>MGHHHHHHAENLYFQGHMLRLSAPGQLDDDLCLLGDVQVPVFLLRLGEASWALVEGGISRDAELVWADLCRWVADPSQVHYWLITHKHYDHCGLLPYLCPRLPNVQVLASERTCQAWKSESAVRVVERLNRQLLRAEQRLPEACAWDALPVRAVADGEWLELGPRHRLQVIEAHGHSDDHVVFYDVRRRRLFCGDALGEFDEAEGVWRPLVFDDMEAYLESLERLQRLPTLLQLIPGHGGLLRGRLAADGAESAYTECLRLCRRLLWRQSMGESLDELSEELHRAWGGQSVDFLPGELHLGSMRRMLEILSRQALPLD[2x];>[2x]MRNDGGFLLWWDGLRSEMQPIHDSQGVFAVLEKEVRRLGFDYYAYGVRHTIPFTRPKTEVHGTYPKAWLERYQMQNYGAVDPAILNGLRSSEMVVWSDSLFDQSRMLWNEARDWGLCVGATLPIRAPNNLLSVLSVARDQQNISSFEREEIRLRLRCMIEL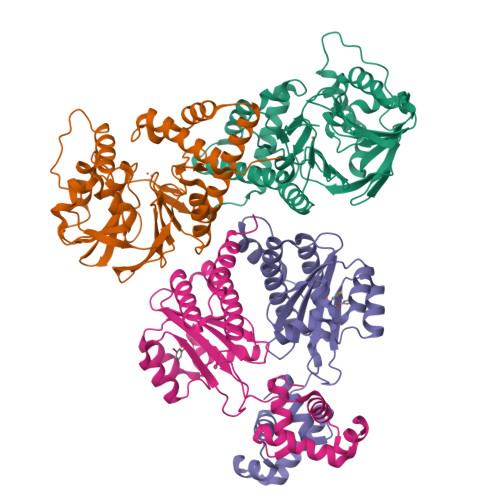LTQKLTDLEHPMLMSNPVCLSHREREILQWTADGKSSGEIAIILSISESTVNFHHKNIQKKFDAPNKTLAAAYAAALGLI> INQVRPKLPLLKILHAAGAQGEMFTVKEVMH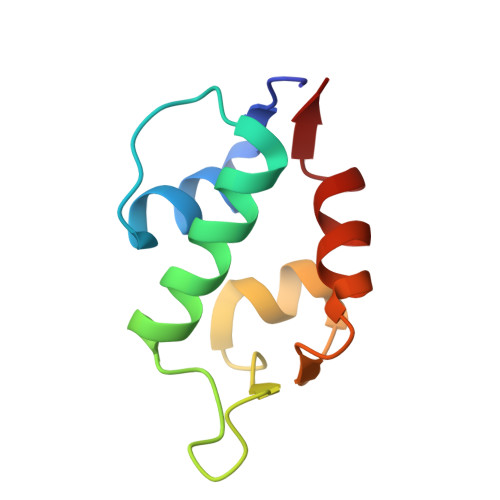YLGQYIMVKQLYDAAAQHMVYCGGDLLGELLGRQSFSVKDPSPLYDMLRKNLVT> GNNYVYIDPTQLPYDHKWEFPRNRLSFGKTLGAGAFGKVVEATAYGLIKSDAAMTVAVKMLKPSAHLTEREALMSELKVLSYLGNHMNIVNLLGACTIGGPTLVITEYCCYGDLLNFLRRKRDSFICSKTSPAIELALDLEDLLSFSYQVAKGMAFLASKNCIHRDLAARNILLTHGRITKICDFGLARDIKNDSNYVVKGNARLPVKWMAPESIFNCVYTFESDVWSYG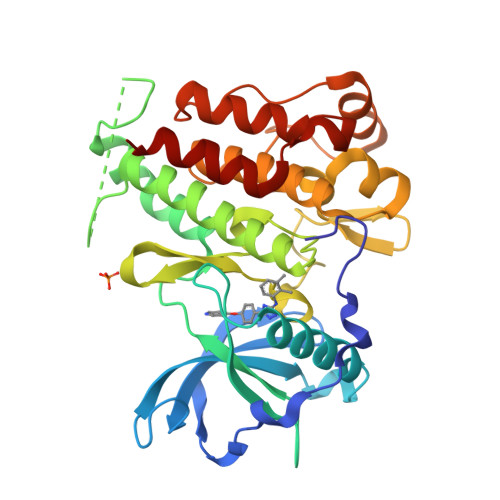IFLWELFSLGSSPYPGMPVDSKFYKMIKEGFRMLSPEHAPAEMYDIMKTCWDADPLKRPTFKQIVQLIEKQIS>[4x]SNHTYRVIEIVGTSPDGVDAAIQG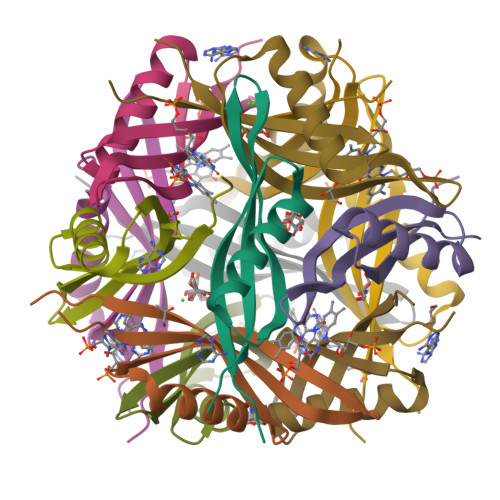GLARAAQTMRALDWFEVQSIRGHLVDGAVAHFQVTMKVGFRLEDS Adeno-Associated Virus (AAV) is a small (~25 nm diameter) non-enveloped single-stranded DNA virus in the Parvoviridae family (genus Dependoparvovirus). The icosahedral proteinaceous shell is composed of three capsid proteins. These proteins (named VP1, VP2 and VP3) share an open reading frame and differ only in their N-terminal residues. We use a high resolution (2.5 Å) cryo-EM structure to analyze details of the molecular interactions that are presumed to be key to efficient infection and are likely to be relevant to serotype-specific tissue tropism.

Gold standard Fourier shell correlation (FSC) curves indicated that a 2.5 Å structure was obtained for the receptor bound dataset and a 2.1 Å structure was obtained for the native virus. These are the highest resolutions achieved for AAV5 structures to date. When comparing both of the reconstructions, there was almost no change in the viral structure upon binding AAVR. Following least-squares superposition, agreement of the new complex structure with the prior structure is reasonable, and excellent compared with the uncomplexed AAV5 structure at 2.1 Å resolution. With high resolution structures of both complex and native virus, interactions can be analyzed at the atomic level.

> SFVDHPPDWLEEVGEGLREFLGLEAGPPKPKPNQQHQDQARGLVLPGYNYLGPGNGLDRGEPVNRADEVAREHDISYNEQLEAGDNPYLKYNHADAEFQEKLADDTSFGGNLGKAVFQAKKRVLEPFGLVEEGAKTAPTGKRIDDHFPKRKKARTEEDSKPSTSSDAEAGPSGSQQLQIPAQPASSLGADTMSAGGGGPLGDNNQGADGVGNASGDWHCDSTWMGDRVVTKSTRTWVLPSYNNHQYREIKSGSVDGSNANAYFGYSTPWGYFDFNRFHSHWSPRDWQRLINNYWGFRPRSLRVKIFNIQVKEVTVQDSTTTIANNLTSTVQVFTDDDYQLPYVVGNGTEGCLPAFPPQVFTLPQYGYATLNRDNTENPTERSSFFCLEYFPSKMLRTGNNFEFTYNFEEVPFHSSFAPSQNLFKLANPLVDQYLYRFVSTNNTGGVQFNKNLAGRYANTYKNWFPGPMGRTQGWNLGSGVNRASVSAFATTNRMELEGASYQVPPQPNGMTNNLQGSNTYALENTMIFNSQPANPGTTATYLEGNMLITSESETQPVNRVAYNVGGQMATNNQSSTTAPATGTYNLQEIVPGSVWMERDVYLQGPIWAKIPETGAHFHPSPAMGGFGLKHPPPMMLIKNTPVPGNITSFSDVPVSSFITQYSTGQVTVEMEWELKKENSKRWNPEIQYTNNYNDPQFVDFAPDSTGEYRTTRPIGTRYLTRPL N-(2-phenylethyl)adenosine 5'-(tetrahydrogen triphosphate) 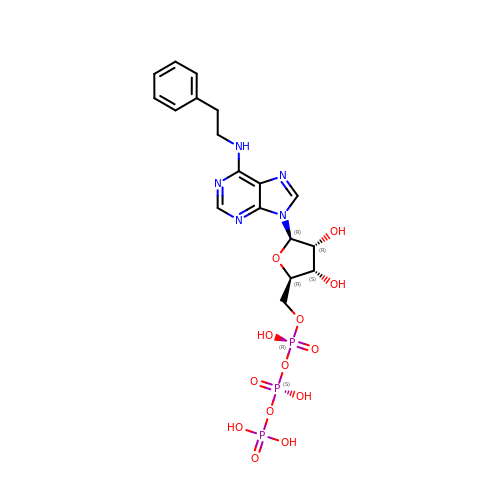| C18 H24 N5 O13 P3 | PSPRNONTFBJUDQ-SCFUHWHPSA-N> MDAAQQGDTTTILMLPWLGYGHLSAFLELAKSLSRRNFHIYFCSTSVNLDAIKPKLPSSFSDSIQFVELHLPSSPEFPPHLHTTNGLPPTLMPALHQAFSMAAQHFESILQTLAPHLLIYDSLQPWAPRVASSLKIPAINFNTTGVFGISQGLHPIHYPHSKFPFSEFVLHNHWKAMYSTADGASTERTRKRGEAFLYCLHASCSVILINSFRELEGKYMDYLSVLLNKKVVPVGPLVYEPNQDGEDEGYSSIKNWLDKKEPSSTVFVSFGSEYFPSKEEMEEIAHGLEASEVNFIWVVRFPQGDNTSGIEDALPKGFLERAGERGMVVKGWAPQAKILKHWSTGGFVSHCGWNSVMESMMFGVPIIGVPMHVDQPFNAGLVEEAGVGVEAKRDPDGKIQRDEVAKLIKEVVVEKTREDVRKKAREMSEILRSKGEEKFDEMVAE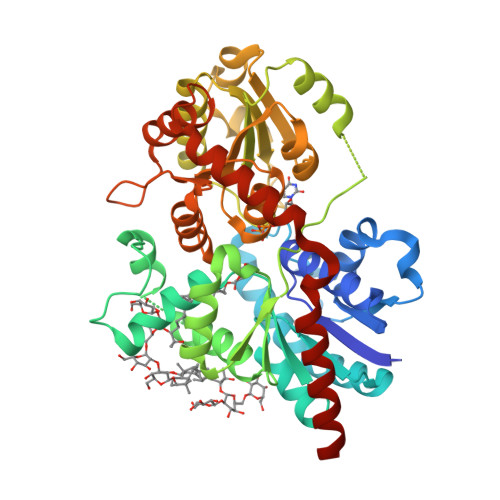ISLLLKIEHHHHHH3-chloro-N-(1,2-oxazol-3-yl)benzamide | C10 H7 Cl N2 O2 | 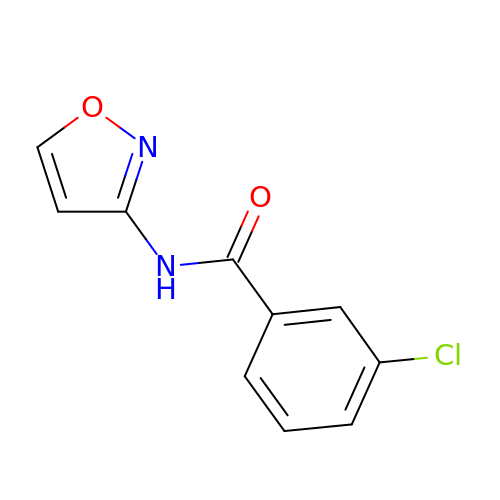YMDSPAORQHWBQI-UHFFFAOYSA-N>[2x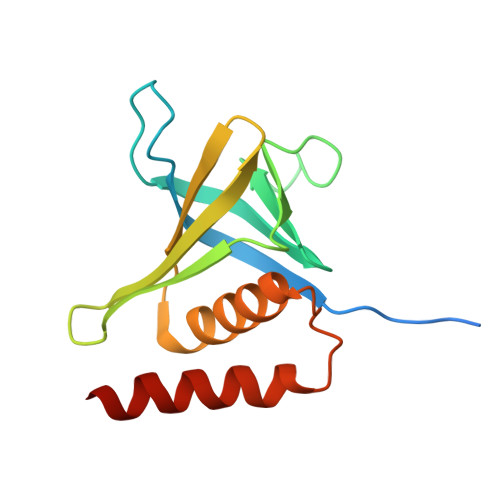]SDLSSGLEVLFQGTDSLTTIPELKDHLRIFRPRKLTLKGYRQYWVVFKDTTLSYYKSQDEAPGDPTQQLNLKGCEVVPDVNVSGQKFCIKLLVPSPEGMSEIYLRCQDEQQYAQWMAACRLASKGRTMADSSYASEVQAILAFLSLQRAG>[2x]GSHMSENFAVATPVRVGIVGTGYAAQRRAEVFRGDRRSQLVSFWGNSEANTAKFADTFGVRPQQSWQALINDPEIDLVLIATINQLHGAIAEAALQAGKHVVLEYPLALTYAMGKKLQQLAREKGKLLHVEHIELLGGVHQAIRQNLGKIGEVFYARYSTIMGQNPAPQRWTYHHQQFGFPLVAALSRISRFTDLFGTVQQVDAQCRFWDQPNPEYFRACLATAYLQFNNGLKAEVIYGKGEVFHQNERIFTLHGDRGTLIFVGETGRLIQGQTETEITVGSRRGLFRQDTEAVLDYLTTGKPLYVDLEASLYALEVADLCAQACGYKVEN

In this study, we used a cyanobacterial BVR from Synechocystis sp. PCC 6803 (Syn BVR)13 as a target for the structural analyses. BVR catalyses the reduction of the C10 double bond (γ-methene bridge) of BV using NAD(P)H to produce BR, a reaction in which the hydride (H−: a proton and two electrons) is donated by NAD(P)H. Syn BVR is composed of 328 residues and shares more than 20% sequence identity with rat and human BVR proteins. Syn BVR consists of two structural domains (N-terminal and C-terminal domains), with the active sites in an obvious cleft between them.

We determined the crystal structure of Syn BVR by the single isomorphous replacement method coupled with anomalous scattering method using an Au-derivative crystal. The structure of apo-Syn BVR was refined at 2.1 Å resolution to R and Rfree values of 0.200 and 0.239, respectively. The asymmetric unit contains two BVR molecules. Although the electron density for apo-Syn BVR was mostly of high quality and continuous, the densities for the N-terminal region (residues 1–8) and C-terminal region (residues 326–328) were poorly defined. Therefore, these residues were not included in the model. The overall topology of Syn BVR is nearly the same as those of the rat and human homologues, with two minor differences: Syn BVR has an additional short α-helix (α2) in the N-terminal domain, and has three additional β-strands in the C-terminal domain. Comparisons between the apo-form and the NADP+-bound form revealed small but significant structural rearrangements upon NADP+ binding: the N-terminal domain shifted ∼1.0 Å in order to expand the active site, and the loop between β5 and a part of helix α6 (residues 129–135) moved ∼2.0 Å away from the nicotinamide ring of the bound NADP+. Because of the steric hindrance configuration of the corresponding site in the apo-form would not able to bind NADP+; accordingly, these movements reflect an ‘induced fit' type of structural change. In the apo-form, the guanidine group of Arg185 in helix α8 formed a hydrogen bond with the carbonyl oxygen of His129 in the loop.> HHHHHHSSENLYFQSLRKDKAEEQTFSWS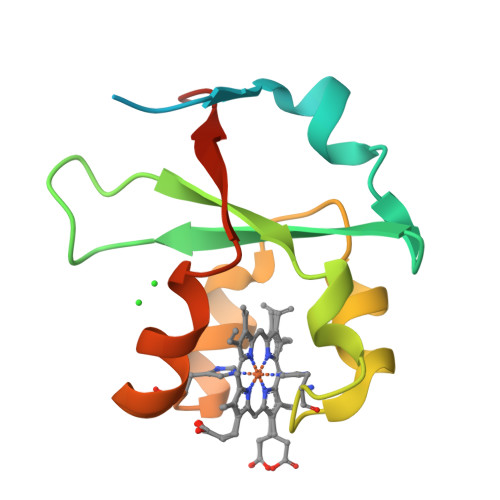EISQHTSANSLWVVVRDKTSPGSPLRVYDVTNFQKTHPGGHLILLKYAGTECSRAFAAVGHSKYAIKRMSQYRIGIAEADNVE> MGSDYKDHDGDYKDHDIDYKDDDDKGSGSLEVLFQGPMDPLNESTVNVYLPDSYLKGVISFSETNAIGSCLLKRPYLKNDNTAKVAIENPVIEHVRLKNAVNSKMKISDYKVVEPVNMQHEIMKNVHSCELTLLKQFLTRSKNISTLKLNMICDWLQLKSTSDDTSILSFIDVEFIPSWVSNWFSNWYNLNKLILEFRREEVIRTGSILCRSLGKLVFIVSSYGCIVKSNKSKRVSFFTYNQLLTWKDVMLSRFNANFCIWVSNSLNENQEGLGLRSNLQGMLTNKLYETVDYMLSLCCNEGFSLVKEFEGFIMSEILRITEHAQFSTRFRNTLLNGLTDQLTKLKNKNRLRVHSTVLENNDYPMYEVVLKLLGDTLRCIKLLINKNLENAAELYYIFRIFGHPMVDERDAMDAVKLNNEITKILRLESLTELRGAFILRIIKGFVDNNKRWPKIKNLKVLSKRWTMYFKAKNYPSQLELSEQDFLELAAIQFEQEFSVPEKTNLEMVLNDKAISPPKRLIWSVYPKNYLPETIKNRYLEETFNASDSLKTRRVLEYYLKDNKFDQKELKSYVVRQEYLNDKEHIVSLTGKERELSVGRMFAMQPGKQRQIQILAEKLLADNIVPFFPETLTKYGDLDLQRIMEIKSELSSIKTRRNDSYNNYIARASIVTDLSKFNQAFRYETTAICADVADELHGTQSLFCWLHLIVPMTTMICAYRHAPPETKGEYDIDKIEEQSGLYRYHMGGIEGWCQKLWTMEAISLLDVVSVKTRCQMTSLLNGDNQSIDVSKPVKLSEGLDEVKADYRLAVKMLKEIRDAYRNIGHKLKEGETYISRDLQFISKVIQSEGVMHPTPIKKVLRVGPWINTILDDIKTSAESIGSLCQELEFRGESIIVSLILRNFWLYNLYMHESKQHPLAGKQLFKQLNKTLTSVQRFFEIKRENEVVDLWMNIPMQFGGGDPVVFYRSFYRRTPDFLTEAISHVDILLKISANIKNETKVSFFKALLSIEKNERATLTTLMRDPQAVGSERQAKVTSDINRTAVTSILSLSPNQLFSDSAIHYSRNEEEVGIIAENITPVYPHGLRVLYESLPFHKAEKVVNMISGTKSITNLLQRTSAINGEDIDRAVSMMLENLGLLSRILSVVVDSIEIPIKSNGRLICCQISRTLRETSWNNMEIVGVTSPSITTCMDVIYATSSHLKGIIIEKFSTDRTTRGQRGPKS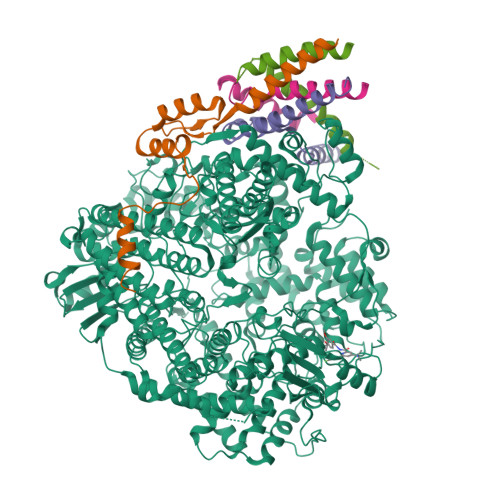PWVGSSTQEKKLVPVYNRQILSKQQREQLEAIGKMRWVYKGTPGLRRLLNKICLGSLGISYKCVKPLLPRFMSVNFLHRLSVSSRPMEFPASVPAYRTTNYHFDTSPINQALSERFGNEDINLVFQNAISCGISIMSVVEQLTGRSPKQLVLIPQLEEIDIMPPPVFQGKFNYKLVDKITSDQHIFSPDKIDMLTLGKMLMPTIKGQKTDQFLNKRENYFHGNNLIESLSAALACHWCGILTEQCIENNIFKKDWGDGFISDHAFMDFKIFLCVFKTKLLCSWGSQGKNIKDEDIVDESIDKLLRIDNTFWRMFSKVMFEPKVKKRIMLYDVKFLSLVGYIGFKNWFIEQLRSAELHEIPWIVNAEGDLVEIKSIKIYLQLIEQSLFLRITVLNYTDMAHALTRLIRKKLMCDNALLTPISSPMVNLTQVIDPTTQLDYFPKITFERLKNYDTSSNYAKGKLTRNYMILLPWQHVNRYNFVFSSTGCKVSLKTCIGKLMKDLNPKVLYFIGEGAGNWMARTACEYPDIKFVYRSLKDDLDHHYPLEYQRVIGELSRIIDSGEGLSMETTDATQKTHWDLIHRVSKDALLITLCDAEFKDRDDFFKMVILWRKHVLSCRICTTYGTDLYLFAKYHAKDCNVKLPFFVRSVATFIMQGSKLSGSECYILLTLGHHNSLPCHGEIQNSKMKIAVCNDFYAAKKLDNKSIEANCKSLLSGLRIPINKKELDRQRRLLTLQSNHSSVATVGGSKIIESKWLTNKASTIIDWLEHILNSPKGELNYDFFEALENTYPNMIKLIDNLGNAEIKKLIKVTGYMLVSKK;>[4x]MSFPEGKDILFMGNEAAKLAEAFQKSLRKPSHKRSQSIIGEKVNTVSETLELPTISRPTKPTILSEPKLAWTDKGGAIKTEAKQTIKVMDPIEEEEFTEKRVLPSSDGKTPAEKKLKPSTNTKKKVSFTPNEPGKYTKLEKDALDLLSDNEEEDAESSILTFEERDTSSLSIEARLESIEEKLSMILGLLRTLNIATAGPTAARDGIRDAMIGIREELIADIIKEAKGKAAEMMEEEMNQRTKIGNGSVKLTEKAKELNKIVEDESTSGESEEEEELKDTQENNQEDDIYQLIMKGENKYFQGHHHHHHH>[2x]GMFQLHERLAADTHKLGESRLCDVLLMNDNTWPWVILVPRVSGIREIYELPNEQQQRLLFESSALSEGMMELFGGDKMNVAALGNMVPQLHLHHIVRY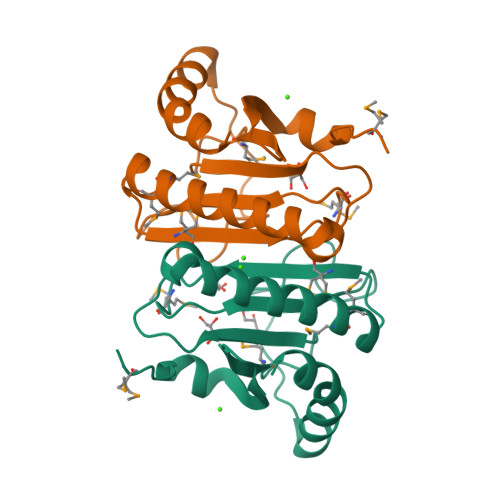QGDPAWPGPVWGKQPPVPYTEEQQASVKAKLQPLLEQLA(2~{R})-~{N}-[(2~{R},3~{S},4~{S},5~{R},6~{R})-5-acetamido-2-methyl-4,6-bis(oxidanyl)oxan-3-yl]-2,3-bis(oxidanyl)propanamide 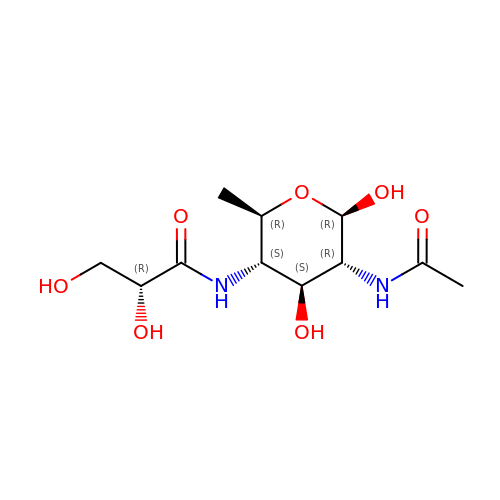| C11 H20 N2 O7 | ZAABMPWLDGVWSW-VQYCFQGSSA-N> MTSLIDLGRYVERTHHGEDTEPRSKRVKIAKPDLSSFQPGSIIKIRLQDFVTYTLTEFNLSPSLNMIIGPNGSGKSTFVCAVCLGLAGKPEYIGRSKKVEDFIKNGQDVSKIEITLKNSPNVTDIEYIDARDETIKITRIITRSKRRSDYLINDYQVSESVVKTLVAQLNIQLDNLCQFLSQERVEEFARLKSVKLLVETIRSIDASLLDVLDELRELQGNEQSLQKDLDFKKAKIVHLRQESDKLRKSVESLRDFQNKKGEIELHSQLLPYVKVKDHKEKLNIYKEEYERAKANLRAILKDKKPFANTKKTLENQVEELTEKCSLKTDEFLKAKEKINEIFEKLNTIRDEVIKKKNQNEYYRGRTKKLQATIISTKEDFLRSQEILAQTHLPEKSVFEDIDIKRKEIINKEGEIRDLISEIDAKANAINHEMRSIQRQAESKTKSLTTTDKIGILNQDQDLKEVRDAVLMVREHPEMKDKILEPPIMTVSAINAQFAAYLAQCVDYNTSKALTVVDSDSYKLFANPILDKFKVNLRELSSADTTPPVPAETVRDLGFEGYLSDFITGDKRVMKMLCQTSKIHTIPVSRRELTPAQIKKLITPRPNGKILFKRIIHGNRLVDIKQSAYGSKQVFPTDVSIKQTNFYQGSIMSNEQKIRIENEIINLKNEYNDRKSTLDALSNQKSGYRHELSELASKNDDINREAHQLNEIRKKYTMRKSTIETLREKLDQLKREARKDVSQKIKDIDDQIQQLLLKQRHLLSKMASSMKSLKNCQKELISTQILQFEAQNMDVSMNDVIGFFNEREADLKSQYEDKKKFVKEMRDTPEFQSWMREIRSYDQDTKEKLNKVAEKYEEEGNFNLSFVQDVLDKLESEIAMVNHDESAVTILDQVTAELRELEHTVPQQSKDLETIKAKLKEDHAVLEPKLDDIVSKISARFARLFNNVGSAGAVRLEKPKDYAEWKIEIMVKFRDNAPLKKLDSHTQSGGERAVSTVLYMIALQEFTSAPFRVVDEINQGMDSRNERIVHKAMVENACAENTSQYFLITPKLLTGLHYHEKMRIHCVMAGSWIPNPSEDPKMIHFGETSNYSFD;> MISTTISGKRPIEQVDDELLSLTAQQENEEQQQQRKRRRHQFAPMTQFNSNTLDEDSGFRSSSDVATADQDNFLEESPSGYIKKVILRNFMCHEHFELELGSRLNFIVGNNGSGKSAILTAITIGLGAKASETN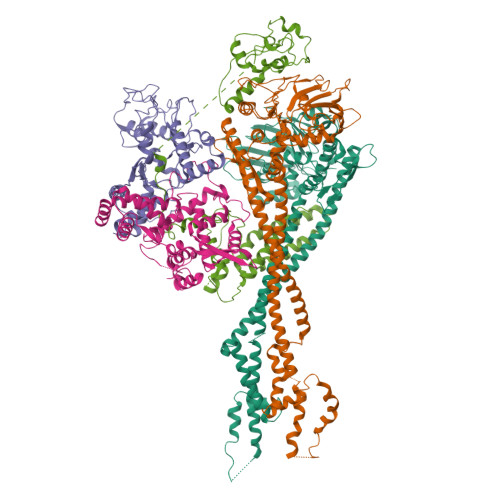RGSSLKDLIREGCYSAKIILHLDNSKYGAYQQGIFGNEIIVERIIKRDGPASFSLRSENGKEISNKKKDIQTVVDYFSVPVSNPMCFLSQDAARSFLTASTSQDKYSHFMKGTLLQEITENLLYASAIHDSAQENMALHLENLKSLKAEYEDAKKLLRELNQTSDLNERKMLLQAKSLWIDVAHNTDACKNLENEISGIQQKVDEVTEKIRNRQEKIERYTSDGTTIEAQIDAKVIYVNEKDSEHQNARELLRDVKSRFEKEKSNQAEAQSNIDQGRKKVDALNKTIAHLEEELTKEMGGDKDQMRQELEQLEKANEKLREVNNSLVVSLQDVKNEERDIQHERESELRTISRSIQNKKVELQNIAKGNDTFLMNFDRNMDRLLRTIEQRKNEFETPAIGPLGSLVTIRKGFEKWTRSIQRAISSSLNAFVVSNPKDNRLFRDIMRSCGIRSNIPIVTYCLSQFDYSKGRAHGNYPTIVDALEFSKPEIECLFVDLSRIERIVLIEDKNEARNFLQRNPVNVNMALSLRDRRSGFQLSGGYRLDTVTYQDKIRLKVNSSSDNGTQYLKDLIEQETKELQNIRDRYEEKLSEVRSRLKEIDGRLKSTKNEMRKTNFRMTELKMNVGKVVDTGILNSKINERKNQEQAIASYEAAKEELGLKIEQIAQEAQPIKEQYDSTKLALVEAQDELQQLKEDINSRQSKIQKYKDDTIYYEDKKKVYLENIKKIEVNVAALKEGIQRQIQNACAFCSKERIENVDLPDTQEEIKRELDKVSRMIQKAEKSLGLSQEEVIALFEKCRNKYKEGQKKYMEIDEALNRLHNSLKARDQNYKNAEKGTCFDADMDFRASLKVRKFSGNLSFIKDTKSLEIYILTTNDEKARNVDTLSGGEKSFSQMALLLATWKPMRSRIIALDEFDVFMDQVNRKIGTTLIVKKLKDIARTQTIIITPQDIGKIADIDSSGVSIHRMRDPERQNNSNFYN;> MEVHEEQVSAPVTGDATAKYLLQYILSARGICHENALILALMRLETDASTLNTEWSIQQWVDKLNDYINAINVKLNLLGYKIIRINHGIGRNAVTLKAKQNFESFEDNTAIRAHNNDYAVLQSIVLPESNRFFVYVNLASTEETKLATRFNQNEIEFMKWAIEQFMISGETIVEGPALETSIIVKEVNRILVAATGDSNLAKWRKFSTFTVGSTNLFQFQELTATDIEDLLLRLCELKWFYRTQEGKFGIDLRCIAELEEYLTSMYNLNTCQNCHKLAIQGVRCGNESCREENEETGENSLSQIWHVDCFKHYITHVSKNCDRCGSSLITEGVYVI;> MSSIDNDSDVDLTEDLAVAKIVKENPVARKMVRYILSRGESQNSIITRNKLQSVIHEAAREENIAKPSFSKMFMDINAILYNVYGFELQGLPSKNNMNAGGNGSNSNTNKSMPEPLGHRAQKFILLNNVPHSKNFDDFKILQSAHTYEELIVTGEYIGDDIASGTSNTLESKLSTDRDLVYKGVLSVILCIVFFSKNNILHQELIKFLETFGIPSDGSKIAILNITIEDLIKSLEKREYIVRLEEKSDTDGEVISYRIGRRTQAELGLESLEKLVQEIMGLEKEQTKSLHDDIIKSIGDSYSI;> MSSTVISRKRRNSTVTEPDSSGETRKQKKSRSDEKSSSSKDGDPQLEFKVLQGYRDLESEMHKGRAQVTRTGDIGVAMDNLNAVDSLFNKVIGIKNNGLFAHDARAMVSISELAQISVRNLKFDDSRSMVNLENIVNSLKRYMLKEHFKLNNIAENRNDLTLAADEQSAADQQEESDGDIDRTPDDNHTDKATSSFKATSMRHSYLQQFSHYNEFSQFNWFRIGALYNTISKNAPITDHLMGPLSIEKKPRVLTQRRRNNDQVGEKITAEKITQHSLNSTQQETTPEQVKKCFKKLSKKLGPEGSINLFKFIIDPNSFSRSIENLFYTSFLIKEGKLLMEHDEEGLPTIKIKQSISHTDSRSKEIERQRRRAAHQNHIIFQMDMPTWRKLIKKYNITSPFLD As the first identified cell fate determinant, Numb transiently forms a basal crescent during mitosis, preferentially segregates to the basal GMC daughter, and then promotes its differentiation to neurons/glia by antagonizing Notch signaling. During NB division, Pon together with Numb is basally localized and is segregated into the basal daughter cell. We found that Numb PTB specifically recognizes the AB motif repeats of its adaptor Pon in a previously unrecognized manner. The multivalent interaction between Numb and Pon can lead to LLPS of the complex, forming condensed, autonomously assembled membrane-lacking compartments both in vitro and in living cells.

Several repeating motifs have been found in Pon1-228: type A “FxNxx[F/L]” motif and type B “NP[F/Y]E[V/I]xR” motif. Proper combination of both motifs dramatically increased the interaction with Numb PTB, whereas the isolated one barely bound to it. For example, Pon fragments containing either B1A2, A2B2, or A3B3 showed significantly enhanced binding avidity to PTB compared with the isolated A or B motifs. To elucidate how combination of A and B motifs can strengthen Pon’s binding to Numb PTB, we solved the crystal structures of Numb PTB in complex with Pon A2B2 or Pon B1A2 peptides. The complex structures revealed that either Pon A2B2 or Pon B1A2 binding led PTB to form a symmetric dimer-of-dimers in either a “head-to-head” or “tail-to-tail” organization. Pon binding could also induce Numb dimerization in solution. Despite of the distinct domain arrangement in the two complexes, the A or B motifs from B1A2 and A2B2 occupied the identical sites on PTB. For example, the bulky aromatic ring of Tyr154B2 (same as Phe120B1) inserts into a hydrophobic pocket formed by the side chains of Tyr87, Val117, and Ile139 from PTB. The side chain of Arg158B2 (same as Arg124B1) forms hydrogen bonds with the backbone carbonyl oxygen of Glu92PTB. By analyzing all the PTB or PTB/ligand structures deposited in the Protein Data Bank, we further found that the newly identified B motif-binding hydrophobic pocket on the Drosophila Numb PTB appears to be present in most of other PTB domains.

> GSKPHQWQADEEAVRSATCSFSVKYLGCVEVFESRGMQVCEEALKVLRQSRRRPVRGLLHVSGDGLRVVDDETKGLIVDQTIEKVSFCAPDRNHERGFSYICRDGTTRRWMCHGFLACKDSGERLSHAVGCAFAVCLERKQ;> KKKKREHACFENPGLNLELPEKQFNPYEVVRSA>[4x]QSASIEAKTVNST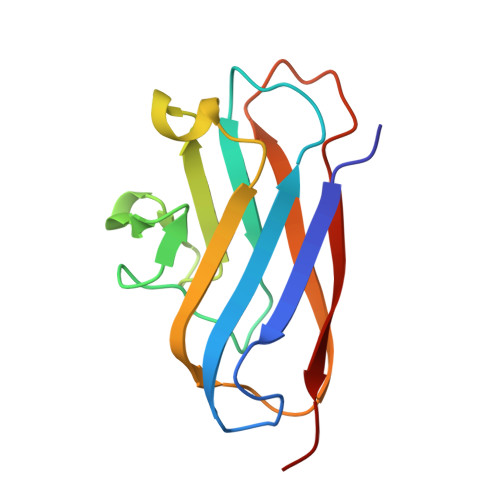KEWTISDIEVTYKPNAVLSLGAVEFQFPDGFHATTRDSVNGRTLKETQILNDGKTVRLPLTLDLLGASEFDLVMVRKTLPRAGTYTIKGDVVNGLGIGSFYAETQLVIDPR PfpI is a ThiJ/DJ-1 family protein from P. aeruginosa that was previously incorrectly annotated as a protease. In summary, our data show that PfpI is a GSH-independent methylglyoxalase. We hypothesize that the primary function of PfpI is in the detoxification of electrophiles such as methylglyoxal (MGO).

Given that the predicted molecular mass of monomeric His6-tagged PfpI is 21.2 kDa, these data indicate that PfpI is likely to be a globular dimer in solution. Purified PfpI crystallized in the space group P 21 21 21 with two molecules in the asymmetric unit. The structure was refined to 1.4 Å resolution with an Rcryst of 0.254 and an Rfree of 0.274. Each PfpI protomer comprised an α/β sandwich containing eight β-strands and eight α-helices. PfpI and its close structural homolog, PH1704 (a protein with proven proteolytic activity from Pyrococcus horikoshii, and which shares 43% amino acid identity (E = 5.2 × 10–38) with PfpI), both possess a “nucleophile elbow”; a distinctive strand–nucleophile–helix motif and a common characteristic of the “α/β hydrolase” protein fold. In PfpI, the nucleophile elbow is comprised of residues 108-118. The nucleophile itself, Cys112, forms part of a constellation of putative catalytic residues, which includes His113, Glu22, and Asp86 from the adjacent protomer. The residues flanking Cys112 (Val-Ile-Cys-His-Gly-Ala) are broadly commensurate with the consensus sequence (small-x-Nuc-x-small-small) conserved in all α/β hydrolases. The X-ray crystal structure of PfpI was similar to that of YhbO, a well-characterized glyoxalase from Escherichia coli. Mutation of Cys112 and His113 in PfpI led to complete loss of methylglyoxalase activity.

>[2x]MTQSLHGKVVAALVTDGFEQVELTGPKKALEDAGATVRILSDKAGEVRGWNHHQPAEAFRVDGTFEDASLDDYDALLLPGGVINSDQIRSLAKAQELAIRAEQASKPVAVICHGAWLLISAGLVQGRTLTSWPSLKDDINNAGGHWVDQEVAVDGKLVSSRKPEDIPAFNRRFIEILAG{[(3,5-dichlorophenyl)amino]methylene}bis(phosphonic acid) | C7 H9 Cl2 N O6 P2 | 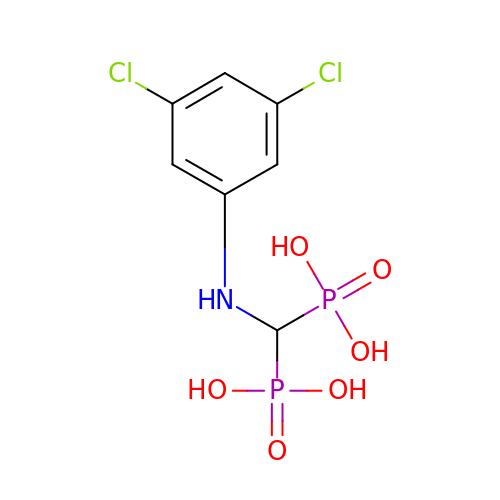ALPQLQJFTUXTFT-UHFFFAOYSA-N>GNSATSADEQPHIGNYRLLKTIGKGNFAKVKLARHILTGKEVAVRIIDKTQLNSSSLQKLFREVRIMKVLNHPNIVKLFEVIETEKTLYLVMEYASGGEVFDYLVAHGRMKEKEARAKFRQIVSAVQYC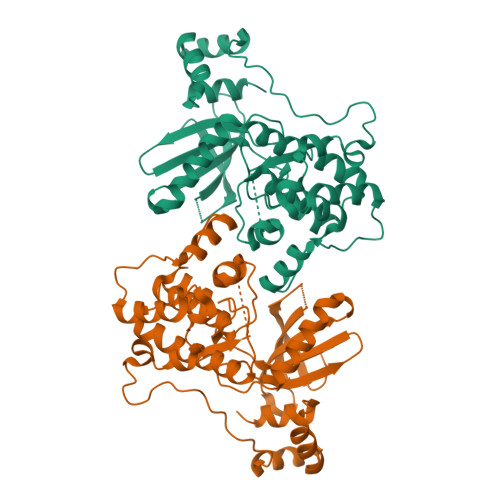HQKFIVHRDLKAENLLLDADMNIKIADFGFSNEFTFGNKLDTFCGSPPYAAPELFQGKKYDGPEVDVWSLGVILYTLVSGSLPFDGQNLKELRERVLRGKYRIPFYMSTDCENLLKKFLILNPSKRGTLEQIMKDRWMNVGHEDDELKPYVEPLPDYKDPRRTELMVSMGYTREEIQDSLVGQRYNEVMATYLLLGYK[2x]> PELPEVETVRRELEKRIVGQKIISIEATYPRMVLTGFEQLKKELTGKTIQGISRRGKYLIFEIGDDFRLISHLRMEGKYRLATLDAPREKHDHLTMKFADGQLIYADVRKFGTWELISTDQVLPYFLKKKIGPEPTYEDFDEKLFREKLRKSTKKIKPYLLEQTLVAGLGNIYVDEVLWLAKI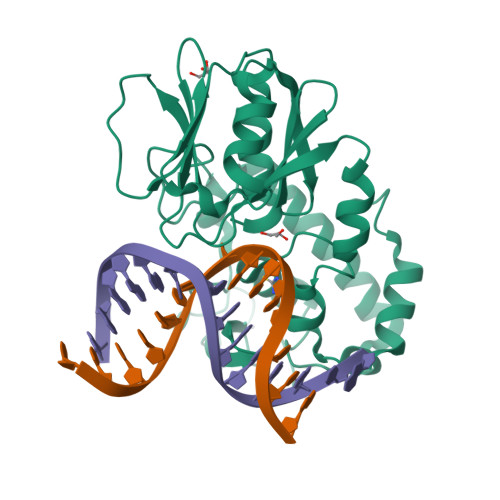HPEKETNQLIESSIHLLHDSIIEILQKAIKLGGSSIRTYSALGSTGKMQNELQVYGKTGEKCSRCGAEIQKIKVAGRGTHFCPVCQQK>[4x]MAVYHMTPPSGWLCDPQRPVTTHGAYQLYYLHSDQNNGPGGWDHASTTDGVAFTHHGTVMPLRPDFPVWSGSAVVDTANTAGFGAGAVVALATQPTDGVRKYQEQYLYWSTDGGFTFTALPDPVIVNTDGRAATTPAEIENAEWFRDPKIHWDTAR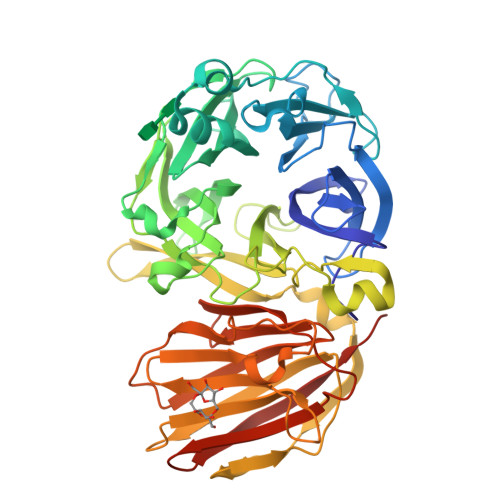GEWVCVIGRLRYAAFYTSPNLRDWTLRRNFDYPNHALGGIECPDLFEITADDGTRHWVLAASMDAYGIGLPMTYAYWTGTWDGEQFHADDLTPQWLDWGWDWYAAVTWPSIDAPETKRLAIAWMNNWKYAARDVPTDASDGYNGQNSIVRELRLARQPGGWYTLLSTPVAALTNYVTATTTLPDRTVDGSAVLPWNGRAYEIELDIAWDTATNVGISVGRSPDGTRHTNIGKYGADLYVDRGPSDLAGYSLAPYSRAAAPIDPGARSVHLRILVDTQSVEVFVNAGHTVLSQQVHFAEGDTGISLYTDGGPAHFTGIVVREIGQAILEHHHHHHHH>[2x]MASYPNSLGSPATVTSTSVPTAKQSSISVAVRVRPFTEAESNRLVKIDNDDVFLGDGCLTSDNNNNNNNSNSNGNGNGNGSSAANSSGASTSRRAIFNTLGGLRKIINVVDDRMLIFDPPETNPLTKMQRNAFPNSFKGSRIREHRFVFDRLFDEDCTQDQVYRNTTQPLLDSVLDGYNATVFAYGATGCGKTHTISGTPE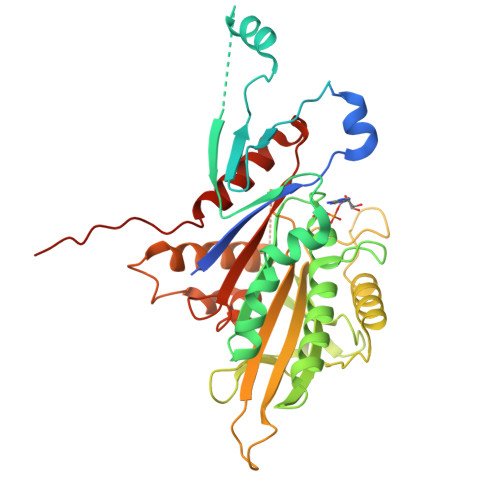DPGVIFLTMKELYNRIEELKDTKIIDISLSYLEIYNETIRDLLNPMTQCKNLVIREDANNKISVSNLSRHRPNSVEEVMQLILEGNKNRTCSPTEANATSSRSHAVLQINVIQKDRTGDITEEHTFATLSIIDLAGSERAAATKNRGARLNEGANINKSLLALGNCINALCDPRRRNHVPYRDSKLTRLLKFSLGGNCKTVMIVCVSPSSQHYDETLNTLKYADRAKEIKTKLIRNLEHHHHHH>MADRFGAFLPHDTSGDVAQLHGIGLQKFGDTWYAYGENKVNGNLFQGVCCYTTTDFIAWRSHGIVLDVQEDGSALAADRIGERPKVLHCPATGKYVMYIHAETPDYGYAHIGVAVADAPTGPFAFQTTITWRGYLSRDIGVFQDEDGSGYIMSEDRDHGTHIYRLADDYLTIVEDVACERATDYPYGLESPTIIKKDGLYYWFGSQLTSWDTNDNKYSTATDLHGPWSEWKLFAPEGAKTYDSQVDIVVPLDDDPYNSEHFLFIGDRWQEHDLGNSPIVQMPISI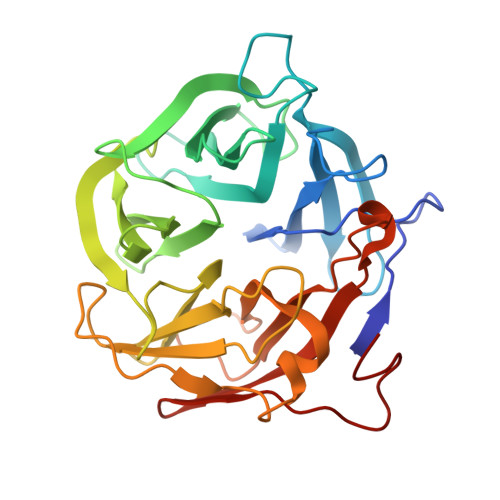ADGVASLTWSDTYEGTTHR[2x]>[4x]MTRRIRIGGAQMGAISRSDSKKEIVDRLIALLRQASEKGCELVVFPELALSTFFPRWYAERDGMDGYFEDGMPNAATLPLFEEARRLGIGFSLGYAELVQEDGRVRRFNTTVLVERNGEIVGKYRKIHLPGHAEYEPERSHQHLEKRYFEVGNTGFQVWDAFGGRVGMAICNDRRWVETYRVMGLQNVELILIGYNTPVNDPLSGEADTLGMFHNHLTMQAGAYQNSTWVVGVAKAGV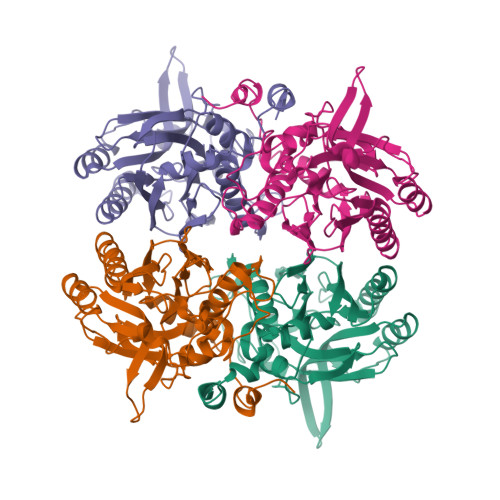EDGHRLMGGSVIVAPTGEIVAQAMTEGDELIVADCDLDLCRYYKSHIFNFAAHRRPEFYQRITSQTGVE>SNALLTGKKILVVDDNIVNRRVAAGALKKFGAEVVCAESGQVALGLLQIPHTFDACFMDIQMPQMDGFEATRQIRMMEKETKEKTNLEWHLPILAMTADVIHATYEECLKS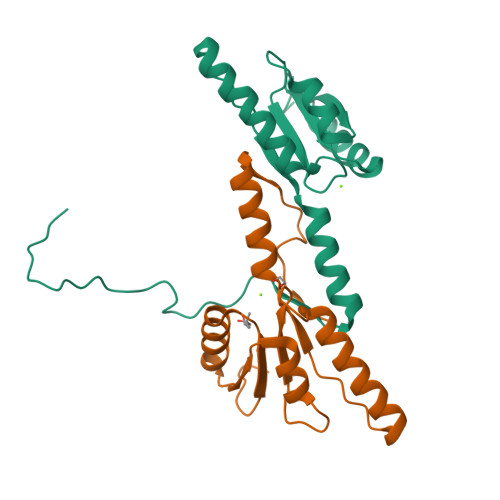GMDGYVSKPFEEENLYKSVAKSFKPNPISPSS[2x]> VGAIMLDGKATRDEIFGDLKQRVAALDAAGRTPGLGTILVGDDPGSQAYVRGKHADCAKVGITSIRRDLPADISTATLNETIDELNANPDCTGYIVQLPLPKHLDENAALERVDPAKDADGLHPTNLGRLVLGTPAPLPCTPRGIVHLLRRYDISIAGAHVVVIGRGVTVGRPLGLLLTRRSENATVTLCHTGTRDLPALTRQADIVVAAVGVAHLLTADMVRPGAAVIDVGVSRTDDGLVGDVHPDVWELAGHVSPNPGGVGPL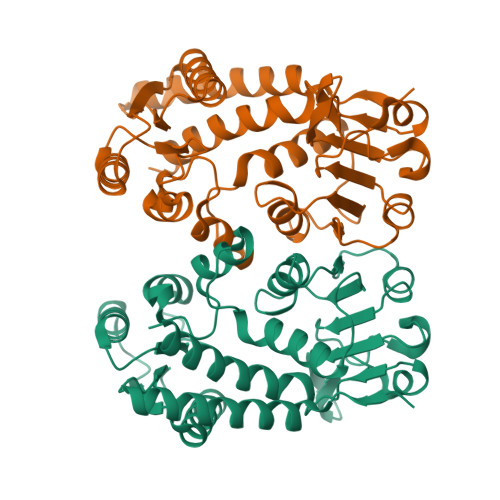TRAFLLTNVVELAERR> SGIVQQQNNLLRAIEAQQHLLQLTVWGIKQLQARILSGGSGGWMEWDREINNYTSLIHSLIEESQNQQEKNEQELLGGSGGSGIVQQQNNLLRAIEAQQHLLQLTVWGIKQLQARILSGGSGGWMEWDREINNYTSLIHSLIEESQNQQEKNEQELLGGSGGSGIVQQQNNLLRAIEAQQHLLQLTVWGIKQLQARIL;> XXTWEAWDRAIAEYAARIEALIRAAQEQQEKNEAAL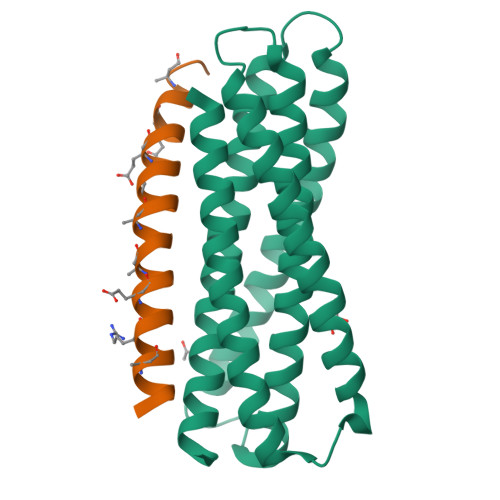RELX> STQLDIVIVLDGSNSIYPWDSVTAFLNDLLERMDIGPKQTQVGIVQYGENVTHEFNLNKYSSTEEVLVAAKKIVQRGGRQTMTALGIDTARKEAFTEARGARRGVKKVMVIVTDGESHDNHRLKKVIQDCEDENIQRFSIAILGSYNRGNLSTEKFVEEIKSIASEPTEKHFFNVSDE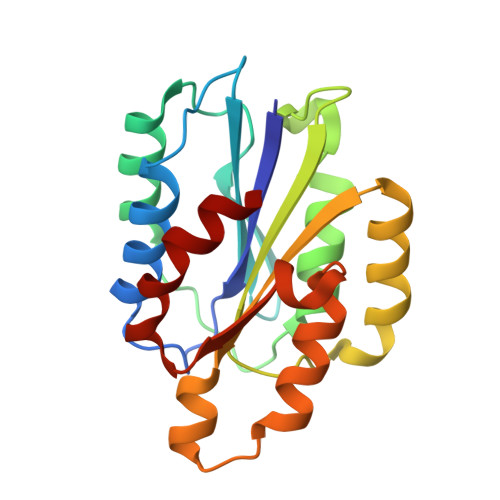IALVTIVKTLGERI> QEITVDEFSNIRENPVTPFNPEPSAPVIDPTAYIDPQASVIGEVTIGANVMVSPMASIRSDEGMPIFVGDRSNVQDGVVLHALETINEEGEPIEDNIVEVDGKEY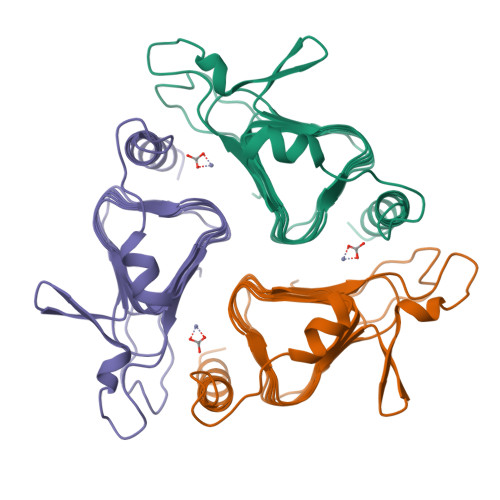AVYIGNNVSLAHQSQVHGPAAVGDDTFIGMQAFVFKSKVGNNCVLEPRSAAIGVTIPDGRYIPAGMVVTSQAEADKLPEVTDDYAYSHTNEAVVYVNVHLAEGYKETS21-NOR-9,10-SECOCHOLESTA-5,7,10(19)-TRIENE-1,3,25-TRIOL, 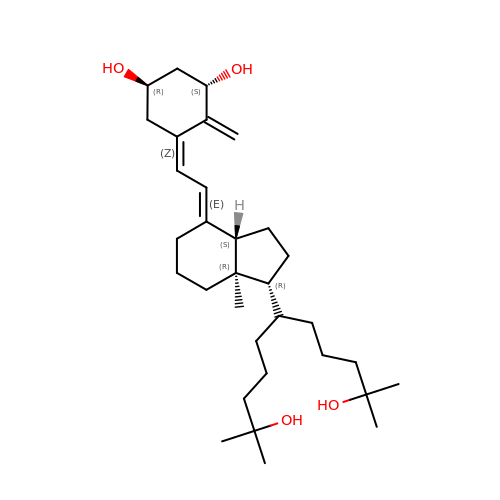20-(4-HYDROXY-4-METHYLPENTYL)-, (1A,3B,5Z,7E) | C32 H54 O4 | WTQXZYVWLNPNEX-LKUPKUSPSA-N>MDHDTEVIVKDFNSILEELTFNSRPII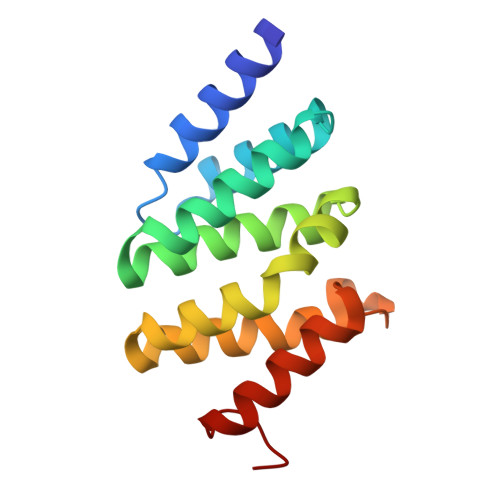TTLTKLAEENISCAQYFVDAIESRIEKCMPKQKLYAFYALDSICKNVGSPYTIYFSRNLFNLYKRTYLLVDNTTRTKLINMFKLWLNPNDTGLPLFEGSALEKIEQFLIKASAAALE[3x]> MNNKTEQGNDAVSGQPSIKGQPVLGKDDAPVTVVEFGDYKCPSCKVFNSDIFPKIQKDFIDKGDVKFSFVNVMFHGKGSRLAALASEEVWKE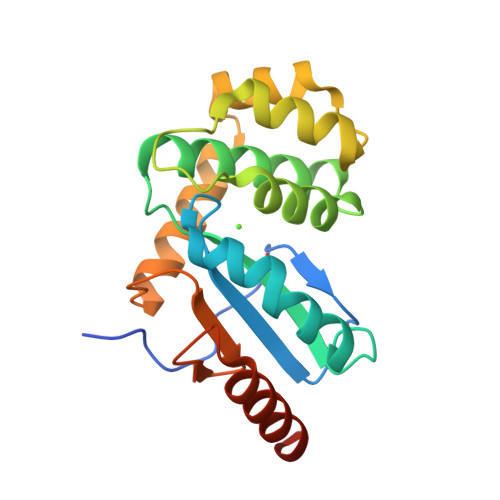DPDSFWDFHEKLFEKQPDTEQEWVTPGLLGDLAKSTTKIKPETLKENLDKETFASQVEKDSDLNQKMNIQATPTIYVNDKVIKNFADYDEIKETIEKELKGKLEHHHHHH> MPVNQSDNNQSEVVTRSATGIKNIVYIEVNDI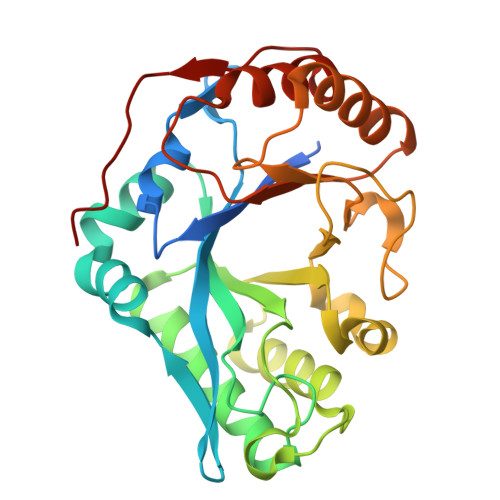NPLNAGSYIMDDAPFFDYVILFAANIRGVGSDATLYNNPNVQYILDHKDTLIKPLQDKGIKVLLGLLGDHTGLGFANMNSAQTEQFATAVANAVSQYGLDGVDFADAWAEYGRNGYPSGSTGSFSNLITALHNKMPGKTITVFNYGYTSELTGVNSYIDYGIYAFFNSPSWSTGFGMPNSKFAPYTINLNSAPSAASAQLYSGQVASKGYGAIGYYDLRANNIVSVLNGVAKGAFKSTCTYDGNSYPKNY> MVTVPDKNPPCPCCGTRVNSVLNLIEHLKVSHGKRGVCFRCAKCGKENSNYHSVVCHFPKCRGPETEKAPAGEWICEVCNRDFTTKIGLGQHKRLAHPAVRNQERIVASQPKETSNRGAHKRCWTKEEEELLIRLEAQFEGNKNINKLIAEHITTKTAKQISDKRRLLSRKPAEEPREEPGTCHHTRRAAASLRTEPEMSHHAQAEDRDNGPGRRPLPGRAAAGGRTMDEIRRHPDKGNGQQRPTKQKSEEQLQAYYKKTLEERLSAGALNTFPRAFKQVMEGRDIKLVINQTAQDCFGCLESISQIRTATRDKKDTVTREKHPKKPFQKWMKDRAIKKGNYLRFQRLFYLDRGKLAKIILDDIECLSCDIPLSEIYSVFKTRWETTGSFKSLGDFKTYGKADNTAFRELITAKEIEKNVQEMSKGSAPGPDGITLGDVVKMDPEFSRTMEIFNLWLTTGKIPDMVRGCRTVLIPKSSKPDRLKDINNWRPITIGSILLRLFSRIVTARLSKACPLNPRQRGFIRAAGCSENLKLLQTIIWSAKREHRPLGVVFVDIAKAFDTVSHQHIIHALQQREVDPHIVGLVSNMYENISTYITTKRNTHTDKIQIRVGVKQGDPMSPLLFNLAMDPLLCKLEESGKGYHRGQSSITAMAFADDLVLLSDSWENMNTNISILETFCNLTGLKTQGQKCHGFYIKPTKDSYTINDCAAWTINGTPLNMIDPGESEKYLGLQFDPWIGIARSGLSTKLDFWLQRIDQAPLKPLQKTDILKTYTIPRLIYIADHSEVKTALLETLDQKIRTAVKEWLHLPPCTCDAILYSSTRDGGLGITKLAGLIPSVQARRLHRIAQSSDDTMKCFMEKEKMEQLHKKLWIQAGGDRENIPSIWEAPPSSEPPNNVSTNSEWEAPTQKDKFPKPCNWRKNEFKKWTKLASQGRGIVNFERDKISNHWIQYYRRIPHRKLLTALQLRANVYPTREFLARGRQDQYIKACRHCDADIESCAHIIGNCPVTQDARIKRHNYICELLLEEAKKKDWVVFKEPHIRDSNKELYKPDLIFVKDARALVVDVTVRYEAAKSSLEEAAAEKVRKYKHLETEVRHLTNAKDVTFVGFPLGARGKWHQDNFKLLTELGLSKSRQVKMAETFSTVALFSSVDIVHMFASRARKSMVM

R2 retrotransposons are sequence-specific mobile elements that insert to the tandemly repeated 28S ribosomal RNA (rRNA) precursor gene locus (the rDNA) and are found within the genomes of multicellular animals including insects, crustaceans, and nonmammalian vertebrates. R2p inserts a cDNA for the mRNA transcribed from the R2 element by nicking one of the two DNA strands of the target site to create a primer for cDNA synthesis directly into the genome. Here, we report high-resolution cryo–electron microscopy structures of two vertebrate A-clade R2 proteins at the initiation of target-primed reverse transcription and after cDNA synthesis and second-strand nicking. The shared R2p core domains include the RT fingers and palm motifs (colored as RT domain) followed by the Thumb, a Linker, the C-terminal zinc-knuckle (ZnK), and the restriction-like endonuclease domain (RLE).

In this work, using cryo–electron microscopy (cryo-EM), we determine structures of an A-clade avian R2p that has optimal transgene insertion activity in human cell PRINT (R2p from the zebrafinch Taeniopygia guttata) as well as a newly isolated testudine (turtle) R2p that is in the Reptilia phylogenetic branch proximal to Aves. We therefore assembled TPRT complexes with PlaMe and TaGu proteins with either Gf-full or Gf-98 RNA. Within Gf-full or Gf-98, only the RNA 3′-terminal 65 nt before the base-paired RNA-primer duplex is visible in our cryo-EM density maps. In addition to the provided primer-template duplex, an added ddTTP was also resolved. A major difference between the PlaMe and TaGu proteins, in comparison to each other, is the disposition of the Spacer, the region that connects the N-terminal DNA binding domains to the NTE motifs. TaGu has a Spacer of ~80 amino acids that could not be resolved in our cryo-EM map, whereas PlaMe has a Spacer of only ~30 amino acids that we partially observe in our structure in contact with the RT core. While the entire PlaMe CTI could be mapped in the cryo-EM density, the density for the part of the TaGu CTI away from the RT domain and the active site RNA:DNA duplex is only visible in our unsharpened cryo-EM map displayed with a low density threshold. In a recent study, the TaGu CTI was inferred to be a disordered loop and, therefore, used as a location for insertion of accessory protein modules. In contrast, our R2p structure and the results from our functional assays recommend against CTI disruption in an avian A-clade R2p used for transgene insertion.> GSFTERQIVVGICSMAKKSKSKPMKEILERISLFKYITVVVFEEEVILNEPVENWPLCDCLISFHSKGFPLDKAVAYAKLRNPFVINDLNMQYLIQDRREVYSILQAEGILLPRYAILNRDPNNPKECNLIEGEDHVEVNGEVFQKPFVEKPVSAEDHNVYIYYPTSAGGGSQRLFRKIGSRSSVYSPESNVRKTGSYIYEEFMPTDGTDVKVYTVGPDYAHAEARKSPALDGKVERDSEGKEVRYPVILNAREKLIAWKVCLAFKQTVCGFDLLRANGQSYVCDVNGFSFVKNSMKYYDD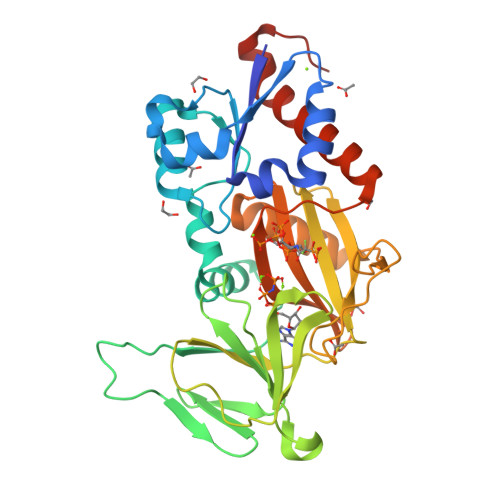CAKILGNIVMRELAPQFHIPWSIPLEAED>[4x]DEEVQEAVERAEELREEAEELIKKARKTGDPELLRKALEALKEAVRAVKEAIKRNPDNEEAVKTAVRLARELLKVAEELKERAEKTGDPRLLLLAAEAIAWAIEAVFLAAKASENTEGALEAARAAVKLAEVAKRIAKLLQRDAKKEGDPELLKLALRALELAVRAVELAIKENPDNEEAVETAKRLAEELRKVAELLEERAKETGDPELQELAKRAKEVADRARELAKKSNPNNSEEQEAARLLELAVEDLKLVLDALEKRR

We set out to design proteins that can switch between two well-defined and fully structured conformations. We reasoned that these goals could be collectively achieved with a “hinge”-like design in which two rigid domains move relative to each other while remaining individually folded. The hinge amplifies small local structural and chemical changes to achieve large global changes while the chemical environment for most residues remains similar throughout the conformational change, avoiding the need for global unfolding. Designing one of the resulting conformations to bind to a target effector couples the conformational equilibrium with target binding.

We solved crystal structures for two designs, cs207 and cs074. For design cs074, the crystal structure of the hinge-peptide complex agrees well with the corresponding state Y design model. For example, cs074 (site pair 1) showed a clear peak between 40 and 50 Å in absence of the peptide, and a peak between 30 and 40 Å in presence of the peptide, and both peaks agree well with the corresponding simulations (top row). In a control experiment using the static parent DHR protein of design cs074, the distance distributions with and without peptide were identical and matched both the simulation for the parent design model, which closely resembles state X, and the experimental distance distribution for state X of cs074. To increase both the absolute distance from N- to C- terminus and the change in termini distance between the two conformational states, we took advantage of the extensibility of repeat proteins and extended hinges cs074, cs221, and cs201 by 1-2 helices on their N and C termini, yielding cs074F, cs221F, and cs201F, respectively (first column). For hinges cs074F and cs221F the distance between the label sites is above the R0 of the dye pair in state X and below R0 in state Y, and hence, acceptor emission upon donor excitation increases upon addition of the corresponding peptides cs074B and cs221B, respectively (second column). We used labeled, extended DHR82, the parent protein for cs074F, as a static control, and observed fluorescence spectra comparable to cs074F but no change in fluorescence upon addition of the peptide. FP based titrations and kinetic characterization using the unlabeled extended hinge cs074F in excess over the TAMRA-labeled peptide cs074B agree well with the corresponding FRET experiments, further supporting the pre-equilibrium model.>[2x]GSMPMYEVQWKVVEESNGNNYSYIDPTQLPYDHKWEFPRNRLSFGKTLGAGAFGKVVEATAQGLIKSDAAMTVAVKMLKPSAHSTEREALMSELKVLSYLGNHENIVNLLGACTHGGPTLVITEYCCYGDLLNFLRRKRDEFVPYKVAPEDLYKDFLTLEHLLSFSYQVAKGMAFLASKNCIHRDLAARNILLTHGNITKICDFGLARDIKNDSNYVDKGNARLPVKWMAPESIFNSVYTFESDVWSYGI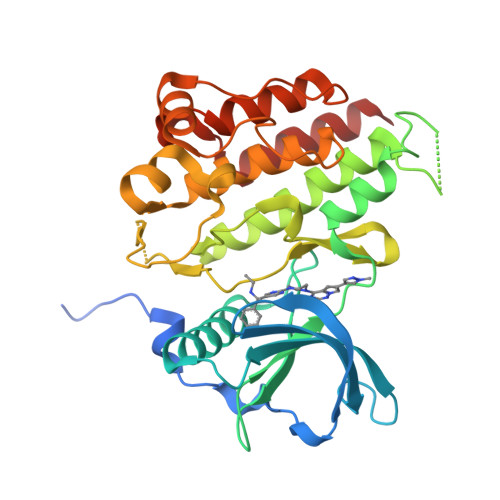FLWELFSLGSSPYPGMPVDSKFYKMIKEGFRMSSPEYAPAEMYDIMKTCWDADPDKRPTFKQIVQDIEKQISESTNH> IVGGYTCGANTVPYQVSLNSGYHFCGGSLINSQWVVSAAHCYKSGIQVRLGEDNINVVEGNEQFISASKSIVHPSYNSNTLNNDIMLIKLKSAASLNSRVASISLPTSCASAGTQCLIS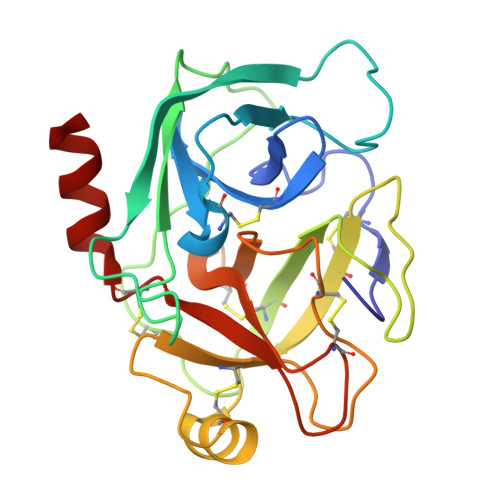GWGNTKSSGTSYPDVLKCLKAPILSTSSCKSAYPGQITSNMFCAGYLEGGKDSCQGDSGGPVVCSGKLQGIVSWGSGCAQKNKPGVYTKVCNYVSWIKQTIASN>[2x]MLESNENRIQIMSTIAKIYRAMSRELN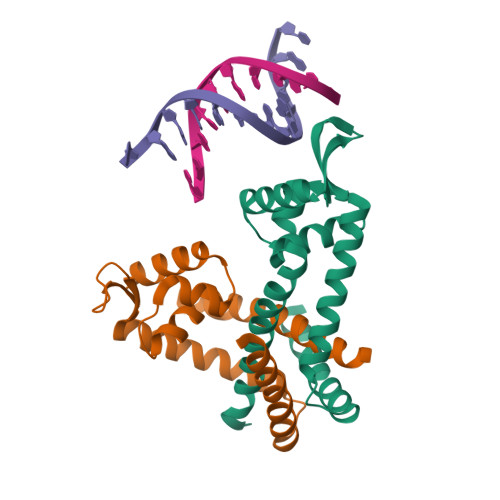RRLGELNLSYLDFLVLRATSDGPKTMAYLANRYFVTQSAITASVDKLEEMGLVVRVRDREDRRKILIEITEKGLETFNKGIEIYKKLANEVTGDLSEDEVILVLDKISKILKRIEEISQ> PKDTIYHAKDAVQATKPDMRKPRLVVFVVGETARADHVSFNGYERDTFPQLAKIDGVTNFSNVTSCGTSTAYSVPCMFSYLGADEYDVDTAKYQENVLDTLDRLGVSILWRDNNSDSKGVMDKLPKAQFADYKSATNNAICNTNPYNECRDVGMLVGLDDFVAANNGKDMLIMLHQMGNHGPAYFKRYDEKFAKFTPVCEGNELAKCEHQSLINAYDNALLATDDFIAQSIQWLQTHSNAYDVSMLYVSDHGESLGENGVYLHGMPN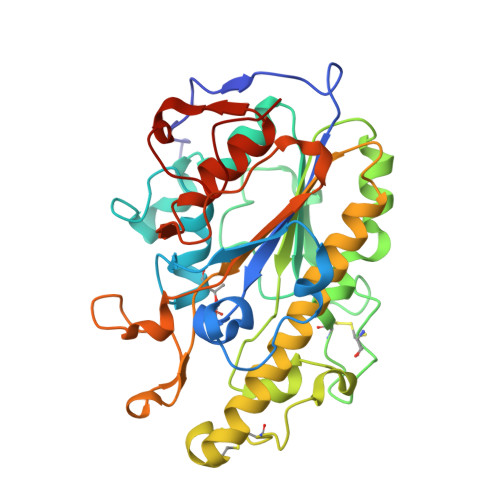AFAPKEQRSVPAFFWTDKQTGITPMATDTVLTHDAITPTLLKLFDVTADKVKDRTAFIRLEHHHHHH> TLLFNEPPEARKPSERWRLYVFKDGEPLNEPLCLHRQSCYLFGRERRIADIPTDHPSCSKQHAVIQYREMEKEKPDGMMGKQVKPYIMDLGSTNKTYINESPI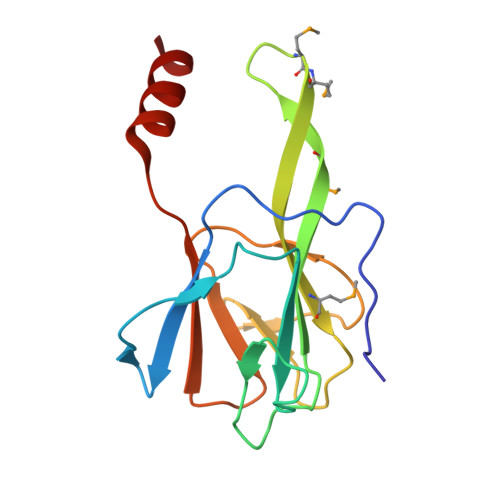EPQRYYELFEKDTIKFGNSSREYVLLHENSAELEHHHHHHHH> GSHMEAVLNELVSVEDLLKFEKKFQSEKAAGSVSKSTQFEYAWCLVRTRYNDDIRKGIVLLEELLPKGSK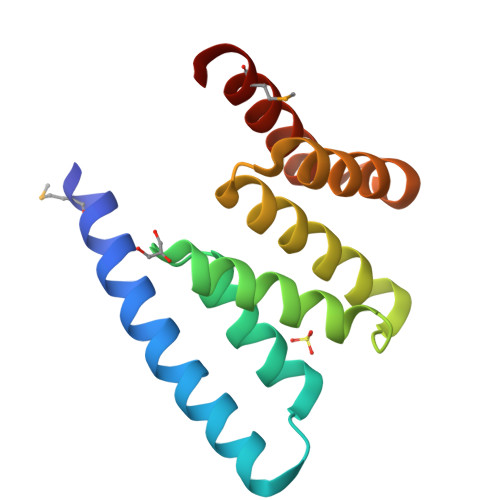EEQRDYVFYLAVGNYRLKEYEKALKYVRGLLQTEPQNNQAKELERLIDKAMKKDGL> GSGSDSFINVINTLGRNDGAKYIGECHSVADLRNTEPTMDGQRIILKQHTAGTLLGGGVFRALIDGTGKTDNNGTVIKTVGGAAWLRVNADRVNPFMFGALGGSNDDTIPVQSCVDSGKATQLTDAHYVSNIQLKYNTSSIYGSGLHYSRLHQLPSATGNCITIKDTCSLIVLDAFGVYGTGAQQGTSFTAGTTGIYVETPSGLSADYPFHTT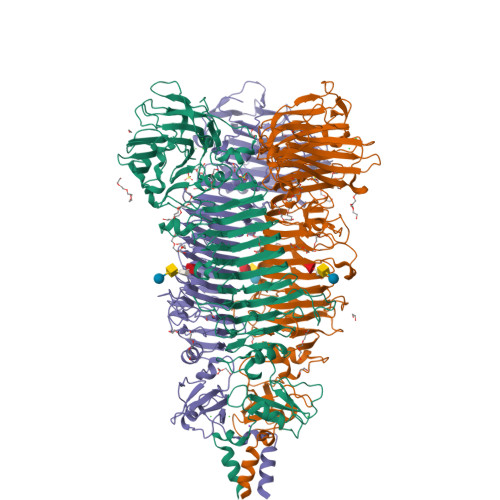ADPRRDLCISKVHIAGFDEYGLNIDSGNFSVTTDSLLVNHINQVGVRCATTDWTWTNIQVNTCGKQCLVLDGCGNGRIIGGKFIWANWQPYGTVGQFPGITINNSQNMVINGIEVQDCGGNGIEISESYSISMNGLNTNRNGINANNTFYNIVFNKSDAVINGFVGLNYAANSGSGANSSAGNFQFLSNDCSVTINGVVETGYMGINFIGDNNIINPTNSDLSINGLVNYSKTGLQTMNETPTFDGVSTTPVYVSVPSSVGQVNGLRLSQANKDKLLYSRTAGPEGITMAAVIVPTISGAEVFNFMAIGSGFSDTSNSLHLQLVIDASGKQTIALLLGGDGTTQILSGDLPNDLKLQSGVPYHIAIGAKPGYFWWSILNIQTGKRIRRSFRGAYLAVPFNSIFGLTSSLTFFSDSNAGGDACSGVGAKVYVGMFSSENDYVASRYYNLINPVDPTKLISYRILDSSI>[4x]GPAAPAQSPAAPDPEASPLAEPPQEQSLAPWSPQTPAPPCSRCFARAIESSRDLLHRIKDEVGAPGIVVGVSVDGKEVWSEGLGYADVEN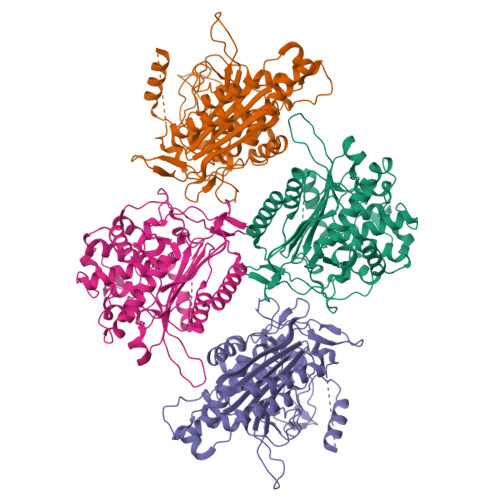RVPCKPETVMRIASISKSLTMVALAKLWEAGKLDLDIPVQHYVPEFPEKEYEGEKVSVTTRLLISHLSGIRHYEKDIKKVKEEKAYKALKMMKENVAFEQEKEGKSNEKNDFTKFKTEQENEAKCRNSKPGKKKNDFEQGELYLREKFENSIESLRLFKNDPLFFKPGSQFLYSTFGYTLLAAIVERASGCKYLDYMQKIFHDLDMLTTVQEENEPVIYNRARFYVYNKKKRLVNTPYVDNSYKWAGGGFLSTVGDLLKFGNAMLYGYQVGLFKNSNENLLPGYLKPETMVMMWTPVPNTEMSWDKEGKYAMAWGVVERKQTYGSCRKQRHYASHTGGAVGASSVLLVLPEELDTETINNKVPPRGIIVSIICNMQSVGLNSTALKIALEFDKDRSD> MEQNLFALSLDDTSSVRGSLLDTKFAQTRVLLSKAMAGGDVLLDEYLYDVVNGQDFRATVAFLRTHVITGKIKVTATTNISDNSGCCLMLAINSGVRGKYSTDVYTICSQDSMTWNPGCKKNFSFTFNPNPCGDSWSAEMISRSRVRMTVICVSGWTLSPTTDVIAKLDWSIVNEKCEPTIYHLADCQNWLPLNRWMGKLTFPQGVTSEVRRMPLSIGGGAGATQAFLANMPNSWISMWRYFRGELHFEVTKMSSPYIKATVTFLIAFGNLSDAFGFYESFPHRIVQFAEVEEKCTLVFSQQEFVTAWSTQVNPRTTLEADGCPYLYAIIHDSTTGTISGDFNLGVKLVGIKDFCGIGSNPGIDGSRLLGAIAQ;> GPVCAEASDVYSPCMIASTPPAPFSDVTAVTFDLINGKITPVGDDNWNTHIYNPPIMNVLRTAAWKSGTI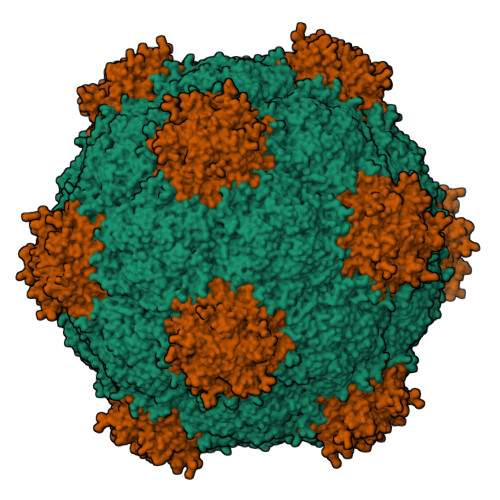HVQLNVRGAGVKRADWDGQVFVYLRQSMNPESYDARTFVISQPGSAMLNFSFDIIGPNSGFEFAESPWANQTTWYLECVATNPRQIQQFEVNMRFDPNFRVAGNILMPPFPLSTETPPLLKFRFRDIERSKRSVMVGHTATAA>[2x]ASNTNLIVNYLPQDMTDRELYALFRAIGPINTCRIMRDYKTGYSYGYAFVDFTSEMDSQRAIKVLNGITVRNKRLKVSYARPGGESIKDTNLYVTNLPRTITDDQLDTIFGK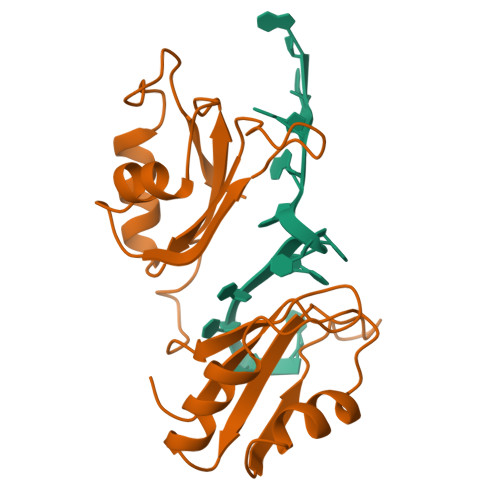YGSIVQKNILRDKLTGRPRGVAFVRYNKREEAQEAISALNNVIPEGGSQPLSVRLA>[4x]LTQELGTAFFQQQQLPAAMADTFLEHLCLLDIDSEPVAARSTSIIATIGPASRSVERLKEMIKAGMNIARLNFSHGSHEYHAESIANVREAVESFAGSPLSYRPVAIALDTKGPEIRTGILQGGPESEVELVKGSQVLVTVDPAFRTRGNANTVWVDYPNIVRVVPVGGRIYIDDGLISLVVQKIGPEGLVTQVENGGVLGSRKGVNLPGAQVDLPGLSEQDVRDLRFGVEHGVDIVFASFVRKASDVAAVRAALGPEGHGIKIISKIENHEGVKRFDEILEVSDGIMVARGDLGIEIPAEKVFLAQKMMIGRCNLAGKPVVCATQMLESMITKPRPTRAETSDVANAV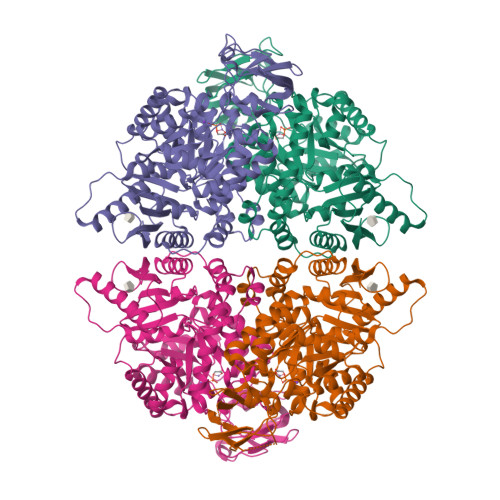LDGADCIMLSGETAKGNFPVEAVKMQHAIAREAEAAVYHRQLFEELRRAAPLSRDPTEVTAIGAVEAAFKCCAAAIIVLTTTGRSAQLLSRYRPRAAVIAVTRSAQAARQVHLCRGVFPLLYREPPEAIWADDVDRRVQFGIESGKLRGFLRVGDLVIVVTGWRPGSGYTNIMRVLSIS> MARTPEEIVKRYKEANIWLRHW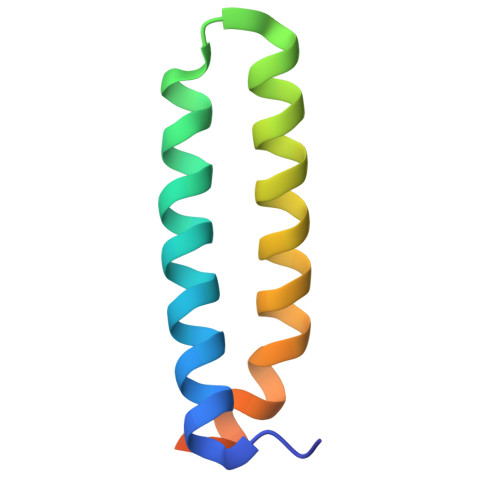KQQIGLAKDEEQREMFTQYYEERVQEIAALEEPYRAALKILNQQESQR> XVDSVYRTRSLGVAAEGIPDQYADGEAARVWQLYIGDTRSRTAEYKAWLLGLLRQHGCHRVLDVACGTGVDSIMLVEEGFSVTSVDASDKMLKYALKERWNRRKEPAFDKWVIEEANWLTLDKDV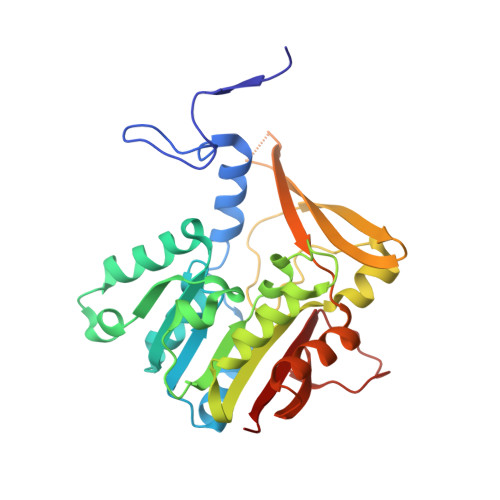PAGDGFDAVICLGNSFAHLPDSKGDQSEHRLALKNIASMVRPGGLLVIDHRNYDYILSTGCAPPGKNIYYKSDLTKDITTSVLTVNNKAHMVTLDYTVQVPGAGRDGAPGFSKFRLSYYPHCLASFTELVQEAFGGRCQHSVLGDFKPYRPGQAYVPCYFIHVLKKTG6-(4-{[3-(2,6-dichlorophenyl)-5-(1-methylethyl)isoxazol-4-yl]methoxy}phenyl)naphthalene-1-carboxylic acid | C30 H23 Cl2 N 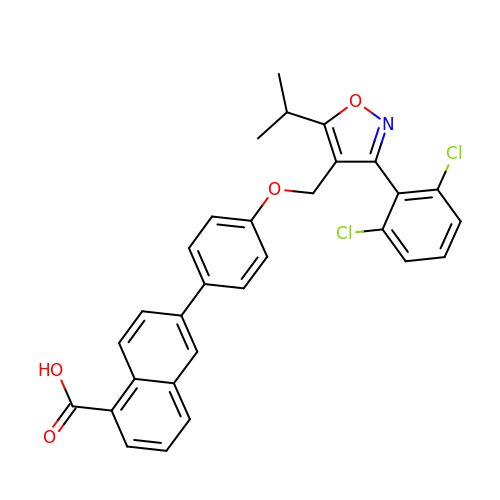O4 | TUOXXRMLFZBSTB-UHFFFAOYSA-N> M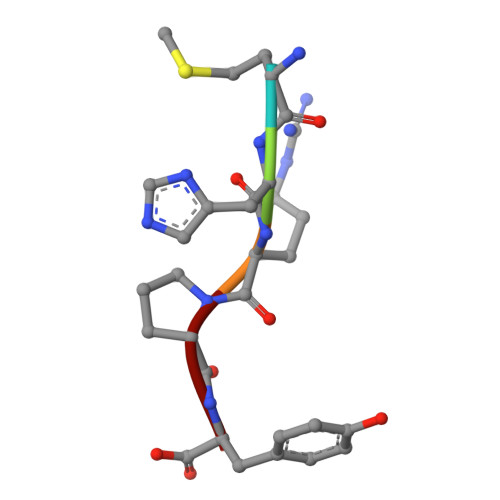HRPY>MAIAQLATEYVFSDFLLKEPTEPKFKGLRLELAVDKMVTCIAVGLPLLLISLAFAQEISIGTQISCFSPSSFSWRQAAFVDSYCWAAVQQKNSLQSESGNLPLWLHKFFPYILLLFAILLYLPPLFWRFAAAPHICSDLKFIMEELDKVYNRAIKAAKSARDLDMRDGACSVPGVTENLGQSLWEVSESHFKYPIVEQYLKTKKNSNNLIIKYISCHLLTLIIILLACIYLGYYFSLSSLSDEFVCSIKSGILRNDSTVPDQFQCKLIAVGIFQLLSVINLVVYVLLAPVVVYTLFVPFRQKTDVLKVYEILPTFDVLHFKSEGYNDLSLYNLFLEENISEVKSYKCLKVLENIKSSGQGIDPMLLLTNLGMIKMDVVDGKTPMSAEMREE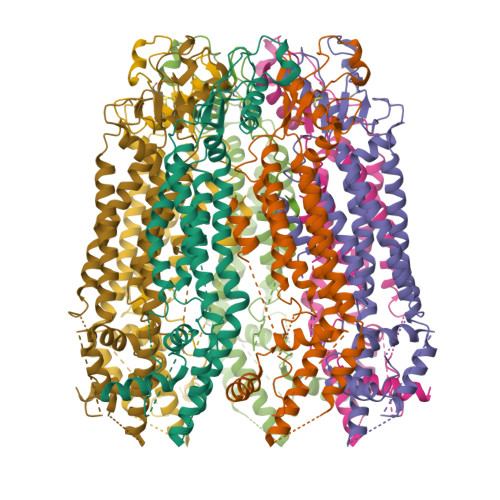QGNQTAELQGMNIDSETKANNGEKNARQRLLDSSC[7x]> MRVLLSVCGTRGDVEIGVALADRLKALGVQTRMCAPPAAEERLAEVGVPHVPVGLPQHMMLQEGMPPPPPEEEQRLAAMTVEMQFDAVPGAAEGCAAVVAVGDLAAATGVRSVAEKLGLPFFYSVPSPVYLASPHLPPAYDEPTTPGVTDIRVLWEERAARFADRYGPTLNRRRAEIGLPPVEDVFGYGHGERPLLAADPVLAPLQPDVDAVQTGAWLLSDERPLPPELEAFLAAGSPPVHIGF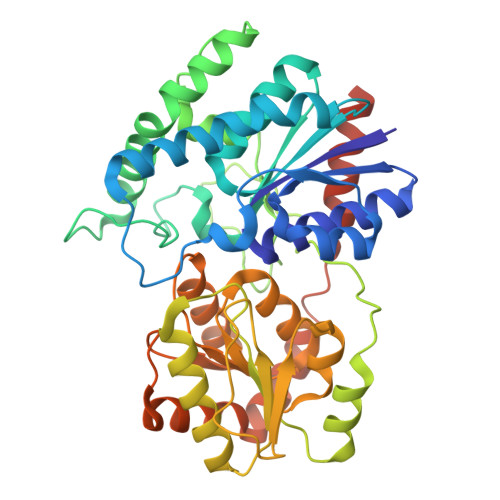GSSSGRGIADAAKVAVEAIRAQGRRVILSRGWTELVLPDDRDDCFAIDEVNFQALFRRVAAVIHHGSAGTEHVATRAGVPQLVIPRNTDQPYFAGRVAALGIGVAHDGPTPTFESLSAALTTVLAPETRARAEAVAGMVLTDGAAAAADLVLAAVGREKPAVPALEHHHHHH Kaposi sarcoma herpes virus (KSHV), a member of the gammaherpesvirinae, has been shown to encode for KsBcl-2, a potent inhibitor of Bcl-2 mediated apoptosis. KsBcl-2 acts by directly engaging host pro-apoptotic Bcl-2 proteins including Bak, Bax and Bok, the BH3-only proteins; Bim, Bid, Bik, Hrk, Noxa and Puma. We also show KsBcl-2 adopts a globular conserved monomeric Bcl-2-fold structure similar to other characterized herpes virus encoded Bcl-2 homologs and binds BH3 motif peptides using the canonical Bcl-2 ligand binding groove. KsBcl-2 lacks any significant shared sequence identity with mammalian Bcl-2 proteins though it does contain a recognizable “NWGR” sequence motif in the BH1 region, which is crucial for pro-survival function of majority of Bcl-2 family proteins.

To establish the structural basis for BH3 ligand engagement by KsBcl-2 we then determined the crystal structure of KsBcl-2 complexes with two of the identified high affinity interactors, Bid and Puma BH3. The KsBcl-2:Bid complex was refined to 1.41 Å, whereas the KsBcl-2:Puma complex was refined to 2.11 Å. Clear and continuous electron density was observed for KsBcl-2 residues 1–146 and Bid residues 79–104 in the KsBcl-2: Bid BH3 complex, as well as KsBcl-2 residues 1–146 and Puma residues 130–155 in the KsBcl-2: Puma BH3 complex. Similarly, in the KsBcl-2: Puma BH3 complex Puma residues I137, L141, M144 and L148 protrude into the four hydrophobic pockets and an extra hydrophobic pocket is occupied by Puma residue W133. Additionally, an ionic interaction is formed by R142PUMA and D79KsBcl-2. However, the expected ionic interaction between pro-survival Bcl-2 proteins and pro-apoptotic BH3 motif ligands between a conserved arginine in the BH1 motif and aspartate of the BH3-motif was surprisingly absent. Additional hydrogen bonds are found between Q132PUMA and Q68KsBcl-2, R142PUMA and V76KsBcl-2, N149PUMA and N83KsBcl-2 as well as between N149BID and Y140KsBcl-2. However, this highly conserved interaction was not seen or is very weak in the KsBcl-2: Puma complex where the closest proximity for this interaction is 5.6 Å. In place of this interaction an alternative salt bridge is observed between D79 KsBcl-2 and R142Puma. Mcl-1:Puma features the hallmark interaction between the conserved Arg residue of the NWGR motif and the well conserved Asp residue of BH3 motif, whereas in KsBcl-2:Puma the NWGR motif is present but this hallmark interaction with the conserved Asp from the BH3 motif is absent.

> GPLGSMDEDVLPGEVLAIEGIFMACGLNEPEYLYHPLLSPIKLYITGLMRDKESLFEAMLANVRFHSTTGINQLGLSMLQVSGDGNMNWGRALAILTFGSFVAQKLSNEPHLRDFALAVLPAYAYEAIGPQWFRARGGWRGLKAYCTQVLT;> EEQWAREIGAQLRRMADDLNAQYERR>[4x]HPETLVKVKDAEDQLGARVGYIELDLNSGKILESFRPEERFPMMSTFKVLLCGAVLSRVDAGQEQLGRRIHYSQNDLVEYSPVTEKHLTDGM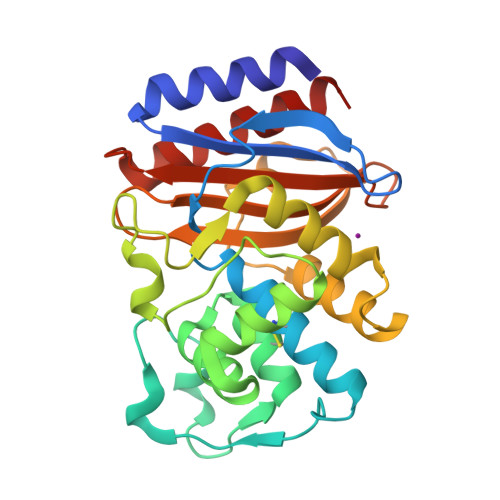TVRELCSAAITMSDNTAANLLLTTIGGPKELTAFLHNMGDHVTRLDRWEPELNEAIPNDERDTTTPAAMATTLRKLLTGELLTLASRQQLIDWMEADKVAGPLLRSALPAGWFIADKSGAGERGSRGIIAALGPDGKPSRIVVIYTTGSQATMDERNRQIAEIGASLIKHW> MIGKNIKSLRKTHDLTQLEFARIVGIS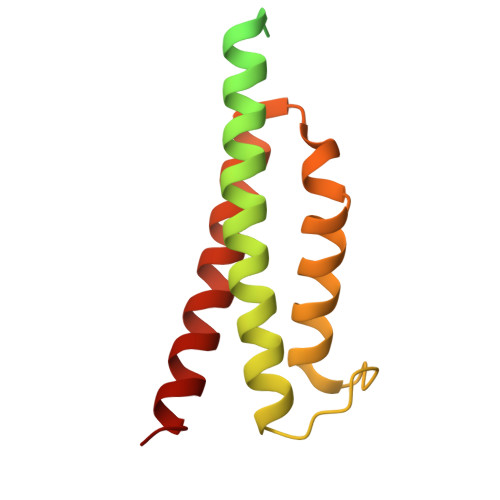RNSLSRYENGTSSVSTELIDIICQKFNVSYVDIVGEDKMLNPVEDYELTLKIEIVKERGANLLSRLYRYQDSQGISIDDESNPWILMSDDLSDLIHTNIYLVETFDEIERYSGYLDGIERMLEISEKRMVA> MGDQPFIPPPQQTALTVNDHDEVTVWNAAPCPMLPRDQVYVRVEAVAINPSDTSMRGQFATPWAFLGTDYAGTVVAVGSDVTHIQVGDRVYGAQNEMCPRTPDQGAFSQYTVTRGRVWAKIPKGLSFEQAAALPAGISTAGLAMKLLGLPLPSPSADQPPTHSKPVYVLVYG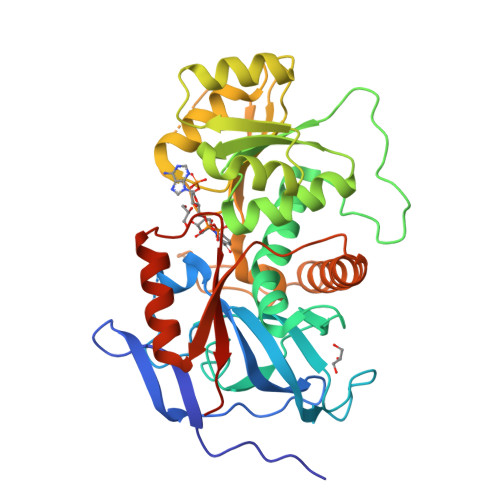GSTATATVTMQMLRLSGYIPIATCSPHNFDLAKSRGAEEVFDYRAPNLAQTIRTYTKNNLRYALDCITNVESTTFCFAAIGRAGGHYVSLNPFPEHAATRKMVTTDWTLGPTIFGEGSTWPAPYGRPGSEEERQFGEDLWRIAGQLVEDGRLVHHPLRVVQGGFDHIKQGMELVRKGELSGEKLVVRLEGPLEHHHHHH> GPHMRYVEIHRNLKGLRKYMAEQAKTNLKLKQRMGDMRREIRKSVGQLTTGGMAANKDKQQKIKSILTEALSNQVESALVDPNNFVVEPRKPVEGATNNDPLLPSIFVYLINIFAKAAISQFINEAGARPETADPVGICVAAILSEPDFLWRGASLIDILIAKFRIVCPVLFGYRGSEKTEQGRQRLGWWKESGQWISEQQHMDRMTGLGAGFAAISLRKFALSKKQNPYPPRFYWMAMAKIVNTPPAEISNTQCVVLKAMVQNYEAKFIEFYGSAAIAALRTALIDFPARAPHKSAAVNSLEVLAQMLKRD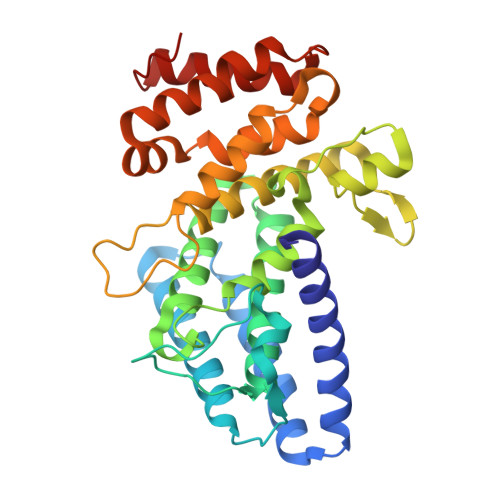TGLDLG> MIALSYKAFLNPYIIEVEKRLYECIQSDSETINKAAHHILSSGGKRVRPMFVLLSGFLNDTQKDDLIRTAVSLELVHMASLVHDDYIDNSDMRRGNTSVHIAFDKDTAIRTGHFLLARALQNIATINNSKFHQIFSKTILEVCFGEFDQMADRFNYPVSFTAYLRRINRKTAILIEASCHLGALSSQLDEQSTYHIKQFGHCIGMSYQI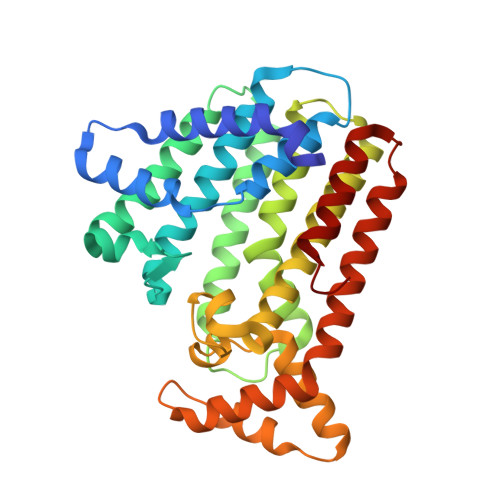IDDILDYTSDEATLGKPVGSDIRNGHITYPLMAAIANLKEQDDDKLEAVVKHLTSTSDDEVYQYIVSQVKQYGIEPAELLSRKYGDKAKYHLSQLQDSNIKDYLEEIHEKMLKRVY αHBs are oligomers of 5 or more α-helical peptides that assemble into coiled-coil structures with central solvent-accessible channels. We targeted two properties of αHBs: oligomeric state, which directly affects the internal diameter of the channel; and the identities of channel-facing residues, which fine tune this dimension and introduce different chemistries. The αHBs are loaded with an environment sensitive dye (in this case, 1,6-diphenyl-1,3,5-hexatriene, DPH) that binds within the channels and fluoresces. Accordingly, challenging the array with analytes leads to differential displacement of the dye across the array to give a fluorescent fingerprint.

Despite the requirements for aliphatic residues at a and d, up to 40% of these can be changed to other side chains without compromising barrel integrity. We introduced mutations at one or two of these sites to generate four groups of αHB: Group I had entirely hydrophobic interiors, but with different sizes and shapes of channel; Groups II and III had polar uncharged or polar charged residues, respectively, at specific points along the channel; and Group IV had aromatic residues installed in their channels. The eleven Group II peptides comprised: single mutants to Cys, His, Asn, Ser or Thr at d sites; and double mutations to His, Asn, Ser or Thr at consecutive a and d sites. Finally, one third of the designs were crystallized and yielded 12 X-ray crystal structures, all of which were open αHBs with fully accessible channels. Focusing on the small molecules, the αSA signal from the more-polar AAs and CHOs is dominated by the polar and charged Group II and III αHBs.

>[2x]XGEIAQALKEIAKALKEIAWALKESAQALKGX> GGGUGCUCAGUACGAG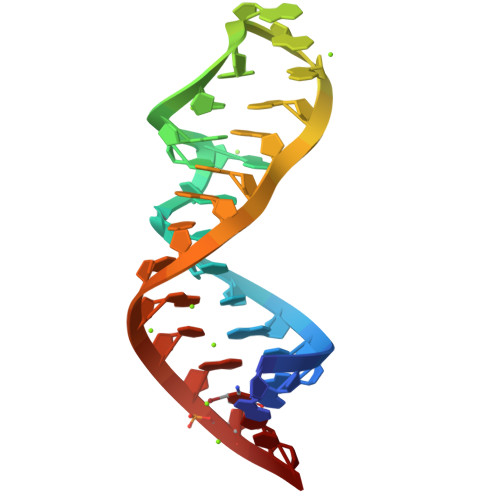AGGAACCGCACCC>[2x]QGHMVSAEGRNRKAVLCQRCGSRVLQPGTALFSRRQLFLPSMRKKPALSDGSNPDGDLLQEHWLVEDMFIFENVGFTKDVGNIKFLVCADCEIGPIGWHCLDDKNSFYVALERVSHE;>MAKTYDYLFKLLLIGDSGVGKT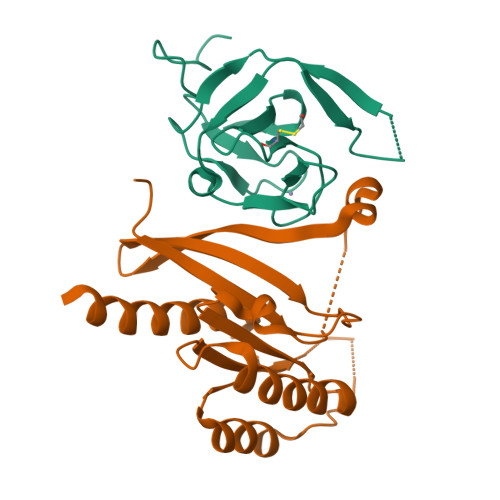CVLFRFSEDAFNSTFISTIGIDFKIRTIELDGKRIKLQIWDTAGQERFRTITTAYYRGAMGIMLVYDITNEKSFDNIRNWIRNIEEHASADVEKMILGNKCDVNDKRQVSKERGEKLALDYGIKFMETSAKANINVENAFFTLARDIKAKMDKNWKATAAG[2x]>SMTGAVCPGSFDPVTLGHLDVFERAAAQFDEVIVAVLINPNKAGMFTVDERIEMIRESTADLPNLRVESGQGLLVDFVRERGLNAIVKGLRTGTDFEYELQ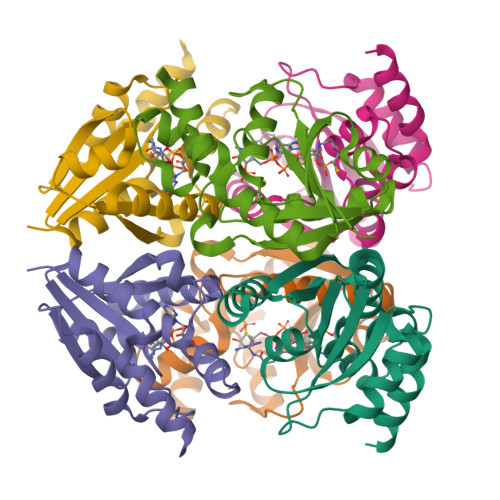MAQMNKHIAGVDTFFVATAPAYSFVSSSLAKEVATYGGDVSALLPASVHQRLLGKLRGQAQ[3x]>[3x]MAQLALQMSSLGVEGEGIWLALGTIGMLLGMLYFIADGLDVQDPRQKEFYVITILIPAIAAASYLSMFFGFGLTEVSLANGRVVDVYWARYADWLFTTPLLLLDIGLLAGASQRDIGALVGIDAFMIVTGLVATLTKVVVARYAFWTISTISMVFLLYYLVAVFGEAVSDADEDTRSTFNALRNIILVTWAIYPVAWLVGTEGLALTGLYGETLLFMVLDLVAKVGFGFILLRSRAIMGGGSEPTPSAQETAADLEHHHHHH

The light-driven proton pumps feature a seven-transmembrane α-helical region with a lysine-bound retinal that serves as a chromophore responsive to light. In this study, wild-type crystal structure of a BR with optical stability under wide pH range from a square halophilic archaeon, Haloquadratum walsbyi (HwBR), was solved in two crystal forms. HwBR could not be classified into any existing subgroup of archaeal BR proteins based on the protein sequence phylogenetic tree, and it showed unique absorption spectral stability when exposed to low pH values. In summary, we characterized the overall important structural and photochemical features in HwBR and in comparison with other known BRs. This study demonstrated how the Arg82–Thr201 hydrogen-bonding network cap gives HwBR a stable optical property in a wide pH range.

In this work, HwBR proteins were crystallized using the in meso method, and the proteins packed into parallel trimeric and antiparallel dimeric crystals diffracted to 1.85 and 2.58 Å, respectively. The structures of the monomers were almost identical and consisted of seven transmembrane α-helices, two β-strands in the BC loops, and a prosthetic group all-trans retinal bound to Lys224 via a Schiff base. The values of root mean square deviation (r.m.s.d.) between monomers of the antiparallel dimer and of the trimer are ∼0.36 Å. The trimeric structure showed that lipids (1-monooleoyl-rac-glycerol, MPG) surrounded each monomer to induce the formation of a self-assembled trimeric structure. We used 30% glycerol as the cryoprotectant when harvesting the crystals. The presence of glycerol improved the resolution from 4 to 1.85 Å. In the structure, one glycerol molecule was found to be bound with chain B. In both structures of HwBR solved in this study, two guanidinium nitrogen atoms of Arg82 located at the BC loop formed hydrogen bonds with the carboxyl group of the main chain of Thr201 in the FG loop in the extracellular region. The location of the Arg82–Thr201 hydrogen-bonding network might shield the retinal-binding pocket from the outside proton equilibrium and protect the protonation condition of both the interior channel and the retinal-binding pocket.> MSDITKIKQEFDKKVAEIQALMKNPQQDSGLLSNSIDFRDQNLIFSNSGGVCTSSKDKIENYPAKGYPYKRG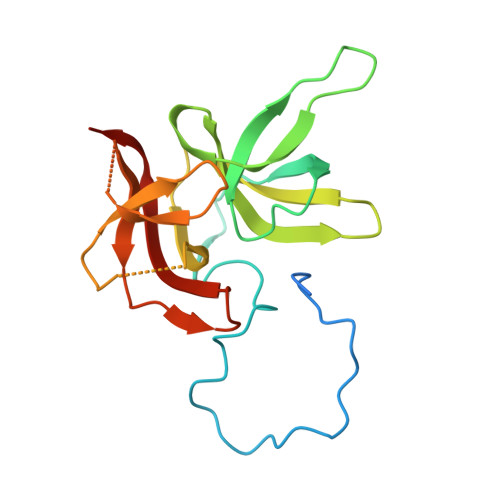VKLSFGDGTTELEVEAGGGDDLYGVCSDIDEFSGMATVIPITNNFTGYLTLKKDGQNGVNPGDKLNFNQHGELEKVTGAQKSVNAIALSKAHKLTEDLFIVLASVFGNRAIKG> SANPYKPKSREVFHPYVPAPEHLPPPAYTTAVLKPMQQFIPKDFYRDMRVDSLRDGVSLGSDFPWNVTHKYRFWRRRKYNIQLDDRFI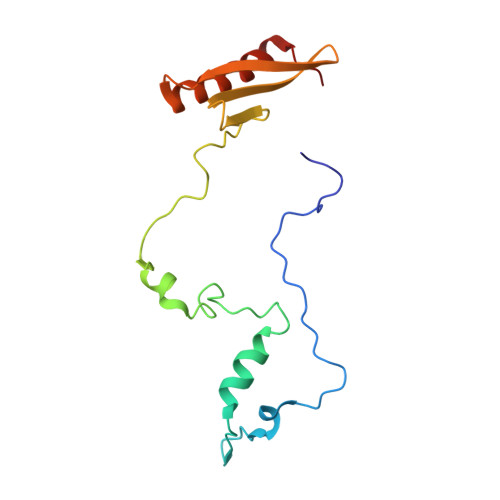RLSPVTGVDYYPRLNVFAVQWREDGQHRIRWFRAAYGLTRAMRAAENFRKTLEATGRVDN> HLICQSGDVLSARYEIVDTLGEGAFGKVVECIDHKAGGRHVAVKIVKNVDRYCEAARSEIQVLEHLNTTDPNSTFRCVQMLEWFEHHGHICIVFELLGLSTYDFIKENGFLPFRLDHIRKMAYQICKSVNFLHSNKLTHTDLKPENILFVQSDYTEAYNPKIKRDERTLINPDIKVVDFGSATYDDEHHSTLVSTRHYRAPEVILALGWSQPCDVWSIGCILIEYYLGFTVFPTHDSKEHLAMMERILGPLPKHMIQKTRKR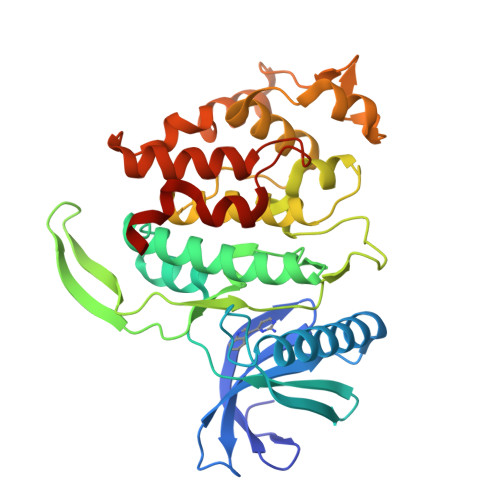KYFHHDRLDWDEHSSAGRYVSRRCKPLKEFMLSQDVEHERLFDLIQKMLEYDPAKRITLREALKHPFFDLLKKSI>[9x]MAQILPIRFQEHLQLQNLGINPANIGFSTLTMESDKFICIREKVGEQAQVVIIDMNDPSNPIRRPISADSAIMNPASKVIALKAGKTLQIFNIEMKSKMKAHTMTDDVTFWKWISLNTVALVTDNAVYHWSMEGESQPVKMFDRHSSLAGCQIINYRTDAKQKWLLLTGISAQQNRVVGAMQLYSVDRKVSQPIEGHAASFAQFKMEGNAEESTLFCFAVRGQAGGKLHIIEVGTPPTGNQPFPKKAVDVFFPPEAQNDFPVAMQISEKHDVVFLITKYGYIHLYDLETGTCIYMNRISGETIFVTAPHEATAGIIGVNRKGQVLSVCVEEENIIPYITNVLQNPDLALRMAVRNNLAGAEELFARKFNALFAQGNYSEAAKVAANAPKGILRTPDTIRRFQSVPAQPGQTSPLLQYFGILLDQGQLNKYESLELCRPVLQQGRKQLLEKWLKEDKLECSEELGDLVKSVDPTLALSVYLRANVPNKVIQCFAETGQVQKIVLYAKKVGYTPDWIFLLRNVMRISPDQGQQFAQMLVQDEEPLADITQIVDVFMEYNLIQQCTAFLLDALKNNRPSEGPLQTRLLEMNLMHAPQVADAILGNQMFTHYDRAHIAQLCEKAGLLQRALEHFTDLYDIKRAVVHTHLLNPEWLVNYFGSLSVEDSLECLRAMLSANIRQNLQICVQVASKYHEQLSTQSLIELFESFKSFEGLFYFLGSIVNFSQDPDVHFKYIQAACKTGQIKEVERICRESNCYDPERVKNFLKEAKLTDQLPLIIVCDRFDFVHDLVLYLYRNNLQKYIEIYVQKVNPSRLPVVIGGLLDVDCSEDVIKNLILVVRGQFSTDELVAEVEKRNRLKLLLPWLEARIHEGCEEPATHNALAKIYIDSNNNPERFLRENPYYDSRVVGKYCEKRDPHLACVAYERGQCDLELINVCNENSLFKSLSRYLVRRKDPELWGSVLLESNPYRRPLIDQVVQTALSETQDPEEVSVTVKAFMTADLPNELIELLEKIV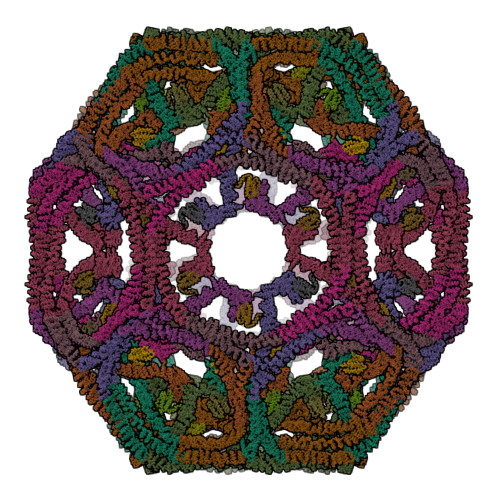LDNSVFSEHRNLQNLLILTAIKADRTRVMEYINRLDNYDAPDIANIAISNELFEEAFAIFRKFDVNTSAVQVLIEHIGNLDRAYEFAERCNEPAVWSQLAKAQLQKGMVKEAIDSYIKADDPSSYMEVVQAANTSGNWEELVKYLQMARKKARESYVETELIFALAKTNRLAELEEFINGPNNAHIQQVGDRCYDEKMYDAAKLLYNNVSNFGRLASTLVHLGEYQAAVDGARKANSTRTWKEVCFACVDGKEFRLAQMCGLHIVVHADELEELINYYQDRGYFEELITMLEAALGLERAHMGMFTELAILYSKFKPQKMREHLELFWSRVNIPKVLRAAEQAHLWAELVFLYDKYEEYDNAIITMMNHPTDAWKEGQFKDIITKVANVELYYRAIQFYLEFKPLLLNDLLMVLSPRLDHTRAVNYFSKVKQLPLVKPYLRSVQNHNNKSVNESLNNLFITEEDYQALRTSIDAYDNFDNISLAQRLEKHELIEFRRIAAYLFKGNNRWKQSVELCKKDSLYKDAMQYASESKDTELAEELLQWFLQEEKRECFGACLFTCYDLLRPDVVLETAWRHNIMDFAMPYFIQVMKEYLTKVDKLDASESLRKEEEQATETQ;>PRTIAEMRKEEMAKEMDPEKLKILEWIEGKERNIRALLSTMHTVLWAGETKWKPVGMADLVTPEQVKKVYRKAVLVVHPDKATGQPYEQYAKMIFMELNDAWSEFENQGQKPLY[9x]> MSKEIPTPYMWSYQPQMGLAAGASQDYSTRMNWLSAGPSMISRVNGVRSHRNQILLEQA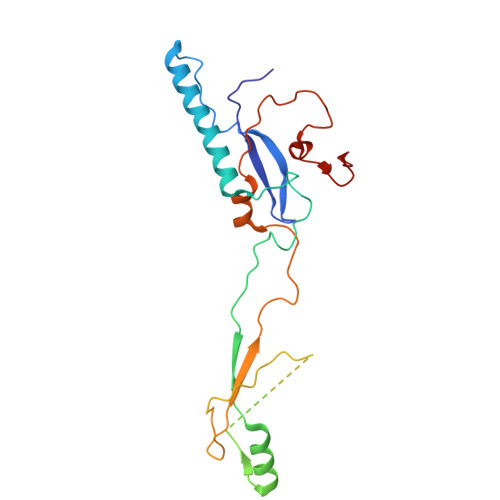AVTSTPRAKLNPRNWPSTLVYQEIPGPTTVLLPRDALAEVRMTNSGVQLAGGASRCPLRPQSGIKTLVIRGRGTQLNDELVSSSIGLRPDGVFQLAGAGRSSFTPNQAYLTLQSSSSEPRSGGIGTLQFVEEFVPSVYFNPFSGSPGLYPDEFIPNFDAVREAVDGYD> GLPTMNTPGSTQFLTSDDFQSPCALPQFDVTPSMNIPGEVKNLMEIAEVDSVVPVNNVQDTTDQMEMFR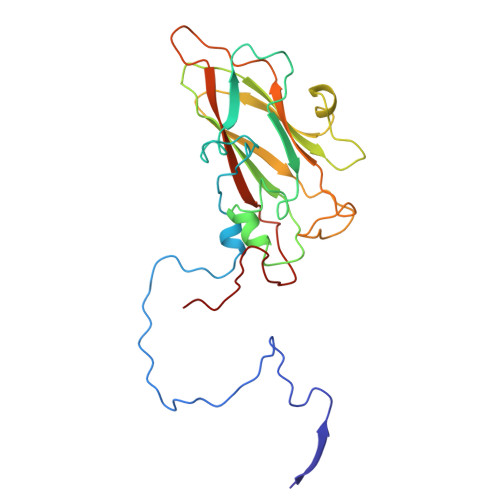IPVTINAPLQQQVFGLRLQPGLDSVFKHTLLGEILNYYAHWSGSMKLTFVFCGSAMATGKFLIAYSPPGANPPKTRKDAMLGTHIIWDIGLQSSCVLCVPWISQTHYRLVQQDEYTSAGYVTCWYQTGMIVPPGTPNSSSIMCFASACNDFSVRMLRDTPFISQDNKLQ>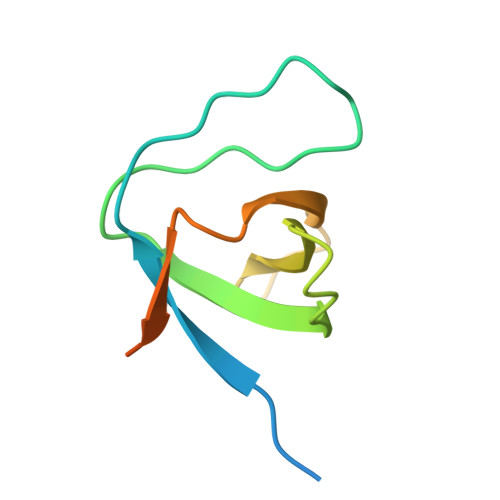 MASMTGGQQMGDARSIVEAMYDYVSEMETDLSFTKGEALIIVENNEGDWWLARKMNSTEVGYIPSNYVKIRDLERGDYKDDDDKKK> GIVLFVDFDYFYAQVEEVLNPSLKGKPVVVCVFSGRFEDSGAVATANYEARKFGVKAGIPIVEAKKILPNAVYLPMRKEVYQQVSSRIMNLLREYSEKIEIASIDEAYLDISDKVRDYREAYNLGLEIKNKILEKEKITVTVGISKNKVFAKIAADMAKPNGIKVIDDEEVKRLIRELDIADVPGIGNITAEKLKKLGINKLVDTLSIEFDKLKGMIGEAKAKYLISLARDEYNEPIRTRVRKSIGRIVTMKRNSRNLEEIKPYLFRAIEES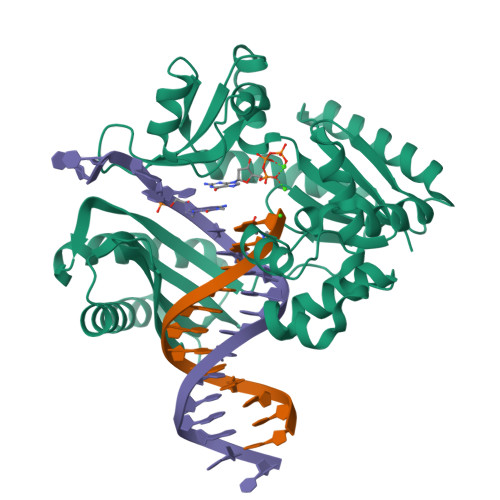YYKLDKRIPKAIHVVAVTEDLDIVSRGRTFPHGISKETAYSESVKLLQKILEEDERKIRRIGVRFSKFI> MAANIPQFPNGQMAMLQQQQQQAQQQAIAANQQYMNVFILNNLRGSGTNLPGTWQAQIPPQQLLSERFQKTHILYTNIMLASNGGDPQRCAVAALNLEKQIFQNAQDKASYDQAMAKKISEVMKRRESNGPALQNQVITDAQRQAQIQQQIQLAQAQQRQQQQLMLNRMAAQGLTQPPQPAFQPMQNPGQVPVIPQQMGINVAVPGMLPNAPSQPQLAMQMGQPRPGAIPVDLNQLSNQDRMRIHEEVMRRVNSTTENSKMQIRQLMQQRLTPAQISEANASGKDLVYLYFQNQVVQVFRATMLQAQEKAQQVAQVQQALLMQQRQGIQGAGMPGVPPQGQVNPALMNALGQQPAISDAPMLGPNLTNEPQMGLLAQQPGQMIVPTNPAAVPGRPVTAGPQLGAIPPQPTPGNPQAPNQTPRPGQLQQPFGMPQVNNPAAAAAAAAAAAAVQQPPQAQPGMRPPGPRTMPGQPGAITTVAGPQPTSQSPAMNTLNAPMRQPPVAMTQATTQPVNPANAPMAGATLNAQFNHQNNARPLSMQGNMNNQAMAGMGAAANMNANNNPMKEFMARLQEQQRATAAAGFQGPKPGQVIGMPGQFPGGPMNALNQPGMFNQNSKPNAMVPPTAQAAALQQQQQQANAADMANIYKIIQTPQGQNMMNNMDIHQMILQEINKHLGGRLPPNITKWAHLRQFLAAQPNALPSEIVQRIMSYQILQFKNFWKRASQPNAVGGIPQPVSNVPVSQFAGMNQPVAPPPGVQVPQSISQVSPQDIEGLRKNPKFANLTDDQLAEWIRKVKQQSFIKKAWEIHNNQSNAAQNQATNSSLIGQQKPGMTVPPTPTTAQPTSSVVQTAQSRPQGPQPTPTPQGPQGVQPQAAQPKPTPSPAANVTTAPPATTGMSAASVQAANIRPSMPQQQQQPAPQPQAPQPPPPQQQQQQQQQQQQQQQQQQQQVPQPPQNSRQAPMDPSPAMATKSLKRPSPDDSAEDTPAQQNITPMQRAPSQAAQVAPNAPNAASGEPPKLSPELQKLRNLASEAQLEVSKEHLQPILMTPADQQETREKIAQVKLKMNQIRSMGLLPKWYYLTNDDNRARQFFRGRFKVVKQFTDGEAMTQLRDTFTITKEELNQYDNLLGSMLRDMMMSRVNQQQAAMMNQQQQTQQQTTQPTPATLANQQAAALRQAQQRVAPPPPKPVQQPPAQQQQPHQPAQPAQQQFQPGVQPTPAPAPEYFGDQRLTA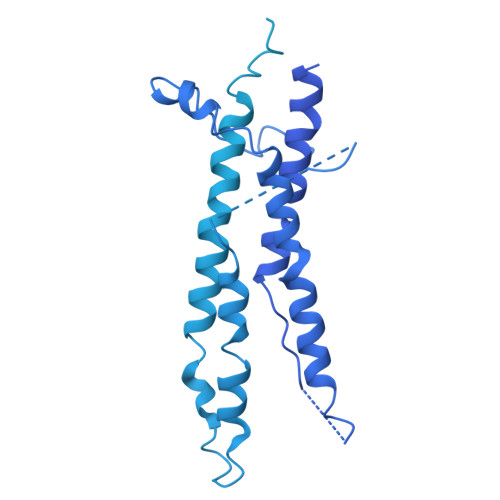ANLVLPPRKKPKVSGNQTSPSANQQLAAGSPQVQALSPVATRKPEPQVKPQAQIPQQQQQQQQQQQQQQQQQQPQAPPAPQFKCPEPGCTSLVAFPSEEALNAHRQEEHLKPAENPLAFMQEQMASVLALDAQGRAKASPKPSGQDVSTPVPTAPPMSASLSKQGQTPRLQAATPMSRNLSMQRQGSASGGKPGENMPTPGKSAGGKGKEGATPQQMEDVWPQGTIDPANLFANLGGTLDAGTATISGSIITDFAAYRSSTPKDTPESSSSSKDSGVSEPNSDINENANLEIDLFWSNIDDGLLMDINNISMDGAAGSMGGSSGNAGGLVDISQFVEDPWGVDSANFSLDDFGRELDKGFGFLDGTLGEGQQESGQGQGQGQPEVMVIE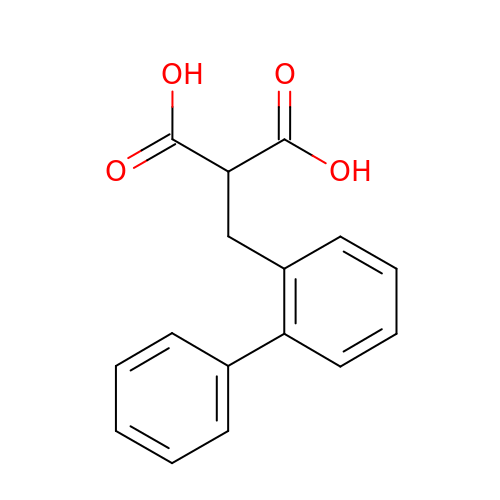[([1,1'-biphenyl]-2-yl)methyl]propanedioic acid | C16 H14 O4 | NRIDIKKHBOBNRS-UHFFFAOYSA-N>[4x]MACHELSALRIAIGEL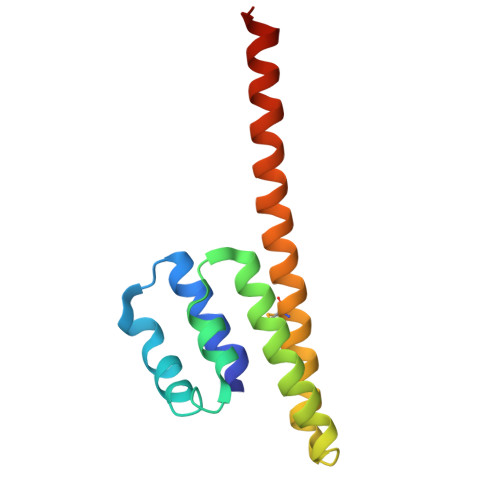LEKEAHDLLHEREELAPVLGQRPELKRLAEAKTLPALEEALREALLHLEERAAQEPEEPYWRGLLLAVEAMEGRLKALRAEAEALYQDLDALHGRLHRLFPRRR> MRPLRPRAALLALLASLLAAPPVAPAEAPHLVQVDAARALWPLRRFWRSTGFCPPLPHSQADPYVLSWDQQLNLAYVGAVPHRGIKQVRTHWLLELVTTRGSTGQGLSYNFTHLDGYLDLLRENQLLPGFELMGSASGHFTDFEDKQQVFEWKDLVSSLARRYIGRYGLAHVSKWNFETWNEPDHHDFDNVSMTMQGFLNYYDACSEGLRAASPALRLGGPGDSFHTPPRSPLSWGLLRHCHDGTNFFTGEAGVRLDYISLHRKGARSSISILEQEKV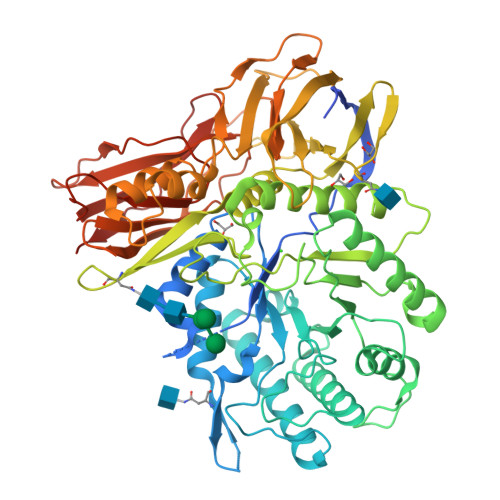VAQQIRQLFPKFADTPIYNDEADPLVGWSLPQPWRADVTYAAMVVKVIAQHQNLLLANTTSAFPYALLSNDNAFLSYHPHPFAQRTLTARFQVNNTRPPHVQLLRKPVLTAMGLLALLDEEQLWAEVSQAGTVLDSNHTVGVLASAHRPQGPADAWRAAVLIYASDDTRAHPNRSVAVTLRLRGVPPGPGLVYVTRYLDNGLCSPDGEWRRLGRPVFPTAEQFRRMRAAEDPVAAAPRPLPAGGRLTLRPALRLPSLLLVHVCARPEKPPGQVTRLRALPLTQGQLVLVWSDEHVGSKCLWTYEIQFSQDGKAYTPVSRKPSTFNLFVFSPDTGAVSGSYRVRALDYWARPGPFSDPVPYLEVPVPRGPPSPGNP> MGSDK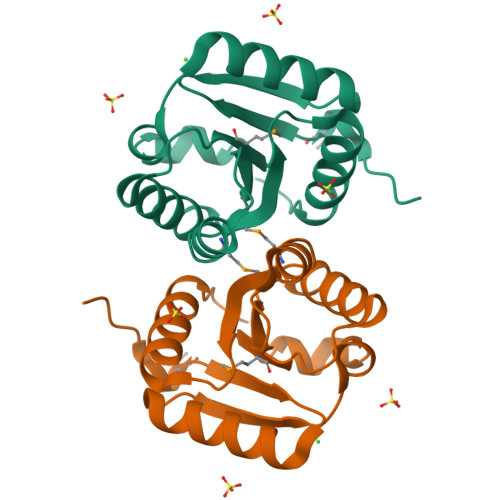IHHHHHHENLYFQGMINILVASEDASRLAHLARLVGDAGRYRVTRTVGRAAQIVQRTDGLDAFDILMIDGAALDTAELAAIEKLSRLHPGLTCLLVTTDASSQTLLDAMRAGVRDVLRWPLEPRALDDALKRAAAQCAQRD>MAALRQPQVAELLAEARRAFREEFGAEPELAVSAPGRVNLIGEHTDYNQGLVLPMALELMTVLVGSPRKDGLVSLLTTSEGADEPQRLQFPLPTAQRSLEPGTPRWANYVKGVIQYYPAAPLPGFSAVVVSSVPLGGGLSSSASLEVATYTFLQQLCPDSGTIAARAQVCQQAEHSFAGMPCGIMDQFISLMGQKGHALLIDCRSLETSLVPLSDPKLAVLITNSNVRHSLASSEYPVRRRQCEEVARALGAASLREVQLEELEAARDLVSKEGFRRARHVVGEIRRTAQAAAALRRGDYRAFGRLMVESHRSLRDDYEVSCPELDQLVEAALAV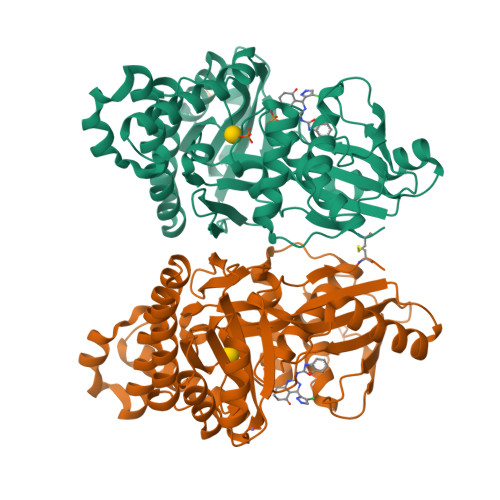PGVYGSRMTGGGFGGCTVTLLEASAAPHAMRHIQEHYGGTATFYLSQAADGAKVLCL[2x]>MTDIINKLQAFADANPQSIAVRHTTDELTYQQLMDESSKLAHRLQGSKKPMILFGHMSPYMIVGMIGAIKAGCGYVPVDTSIPEDRIKMIINKVQPEFVFNTTDESFESLEGEVFTIEDIKTSQDPVIFDSQIKDNDTVYTIFTSGSTGEPKGVQIEYASLVQFTEWMLELNKSGNKQQWLNQAPFSFDLSVMAIYPCLASGGTLNLVDKNMINKPKLLNEMLTATPINIWVSTPSFMEMCLLLPTLNEEQYGSLNEFFFCGEILPHRAAKALVSRFPSATIYNTYGP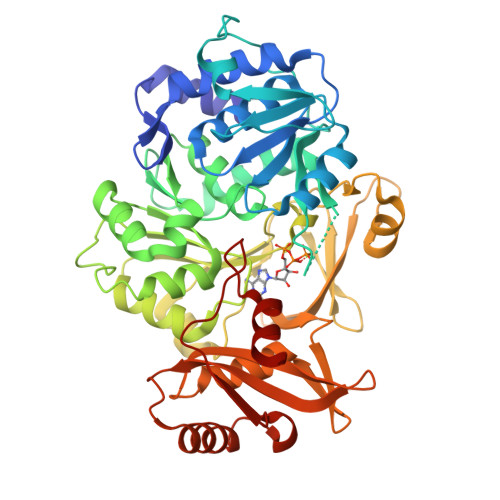TEATVAVTSIQITQEILDQYPTLPVGVERLGARLSTTDDGELVIEGQSVSLGYLKNDQKTAEVFNFDDGIRTYHTGDKAKFENGQWFIQGRIDFQIKLNGYRMELEEIETQLRQSEFVKEAIVVPVYKNDKVIHLIGAIVPTTEVTDNAEMTKNIKNDLKSRLPEYMIPRKFEWMEQLPLTSNGKIDRKKIAEVING[4x]>[6x]ELKILEIIKEAIELGASDIHLTAGAPPAVRIDGYIKFLKDFPRLTPEDTQ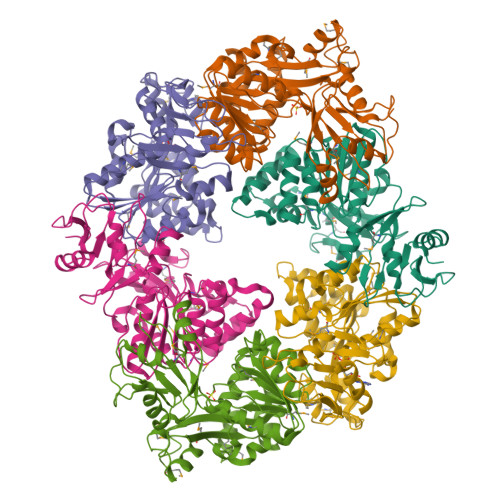KLAYSVMSEKHRQKLEENGQVDFSFGVRGVGRFRANVFYQRGSVAAALRSLPAEIPEFKKLGLPDKVLELCHRKMGLILVTGPTGSGKSTTIASMIDYINQTKSYHIITIEDPIEYVFKHKKSIVNQREVGEDTKSFADALRAALREDPDVIFVGEMRDLETVETALRAAETGHLVFGTLHTNTAIDTIHRIVDIFPLNQQEQVRIVLSFILQGIISQRLLPKIGGGRVLAYELLIPNTAIRNLIRENKLQQVYSLMQSGQAETGMQTMNQTLYKLYKQGLITLEDAMEASPDPKELERMIRGGRLEHHHHHH> AAQTNAPWGLARISSTSPGTSTYYYDESAGQGSCVYVIDTGIEASHPEFEGRAQMVKTYYYSSRDGNGHGTHCAGTVGSRTYGVAKKTQLFGVKVLDDNGSGQYSTIIAGMDFVASDKNNRNCPKGVVASLSLGGGYSSSVNSAAAR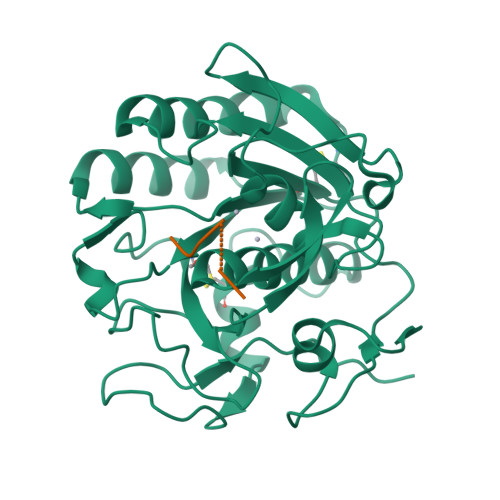LQSSGVMVAVAAGNNNADARNYSPASEPSVCTVGASDRYDRRSSFSNYGSVLDIFGPGTSILSTWIGGSTRSISGTSMATPHVAGLAAYLMTLGKTTAASACRYIADTANKGDLSNIPFGTVNLLAYNNYQA;> PAPFPAX> MSAQGDCEFLVQRARELVPQDLWAAKAWLITARSLYPADFNIQYEMYTIERNAERTATAGRLLYDMFVNFPDQPVVWREISIITSALRNDSQDKQTQFLRSLFETLPGRVQCEMLLKVTEQCFNTLERSEMLLLLLRRFPETVVQHGVGLGEALLEAETIEEQESPVNCFRKLFVCDVLPLIINNHDVRLPANLLYKYLNKAAEFYINYVTRSTQIENQHQGAQDTSDLMSPSKRSSQKYIIEGLTEKSSQIVDPWERLFKILNVV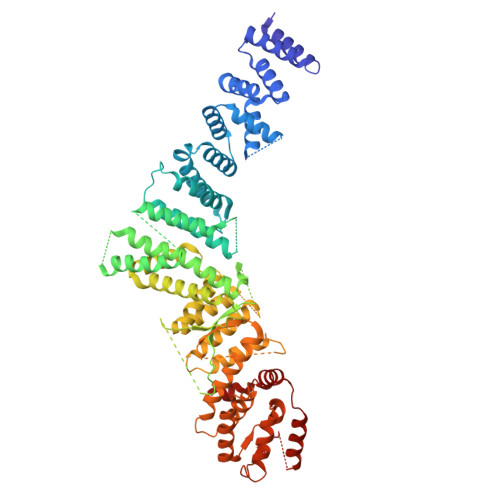GMRCEWQMDKGRRSYGDILHRMKDLCRYMNNFDSEAHAKYKNQVVYSTMLVFFKNAFQYVNSIQPSLFQGPNAPSQVPLVLLEDVSNVYGDVEIDRNKHIHKKRKLAEGREKTMSSDDEDCSAKGRNRHIVVNKAELANSTEVLESFKLARESWELLYSLEFLDKEFTRICLAWKTDTWLWLRIFLTDMIIYQGQYKKAIASLHHLAALQGSISQPQITGQGTLEHQRALIQLATCHFALGEYRMTCEKVLDLMCYMVLPIQDGGKSQEEPSKVKPKFRKGSDLKLLPCTSKAIMPYCLHLMLACFKLRAFTDNRDDMALGHVIVLLQQEWPRGENLFLKAVNKICQQGNFQYENFFNYVTNIDMLEEFAYLRTQEGGKIHLELLPNQGMLIKHHTVTRGITKGVKEDFRLAMERQVSRCGENLMVVLHRFCINEKILLLQTLT>MTETLPPVTESAVALQAE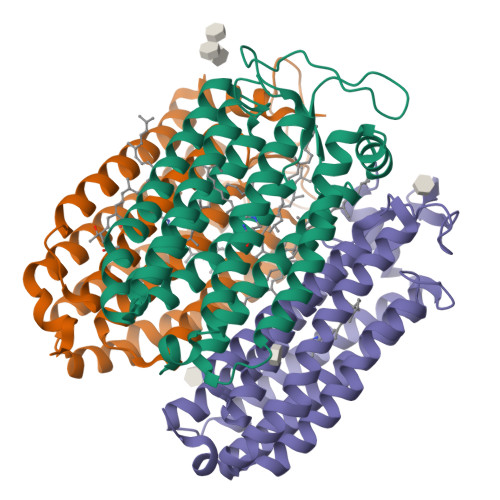VTQRELFEFVLNDPLLASSLYINIALAGLSILLFVFMTRGLDDPRAKLIAVSTILVPVVSIASYTGLASGLTISVLEMPAGHFAEGSSVMLGGEEVDGVVTMWGRYLTWALSTPMILLALGLLAGSNATKLFTAITFDIAMCVTGLAAALTTSSHLMRWFWYAISCACFIVVLYILLVEWAQDAKAAGTADIFSTLKLLTVVMWLGYPIVWALGVEGVAVLPVGYTSWAYSALDIVAKYIFAFLLLNYLTSNEGVVSGSILDVPSASGAPADD[3x]> GMPTLEMPVAAVLDSTVGSSEALPDFTSDRYKDAYSRINAIVIEGEQEAHDNYIAIGTLLPDHVEELKRLAKMEMRHKKGF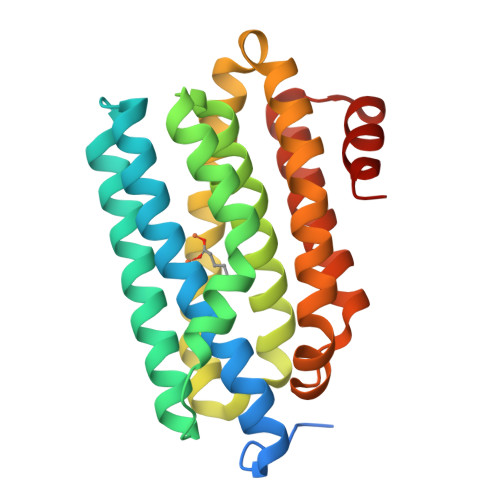TACGKNLGVEADMDFAREFFAPLRDNFQTALGQGKTPTCLLIQALLIEAFAISFYHTYIPVSDPFARKITEGVVKDEYTHLNYGEAWLKANLESCREELLEANRENLPLIRRMLDQVAGDAAVLQMDKEDLIEDFLIAYQESLTEIGFNTREITRMAAAALVS> SNASKEKREKLEAYQHLFYLLQTNPTYLAKLIFQMPQNKSTKFMDSVIFTLYNYASNQREEYLLLRLFKTALQEEIKSKVDQIQEIVTGNPTVIKMVVSFNRGARGQNALRQILAPVVKEIMDDKSLNIKTDPVDIYKSWVNQMESQTGEASKLPYDVTPEQALAHEEVKTRLDSSIRNMRAVTDKFLSAIVSSVDKIPYGMRFIAKVLKDSLHEKFPDAGEDELLKIIGNLLYYRYMNPAIVAPDAFDIIDLSAGGQLTTDQRRNLGSIAKMLQHAASNKMFLGDNAHLSIINEYLSQSYQKFRRFFQTAC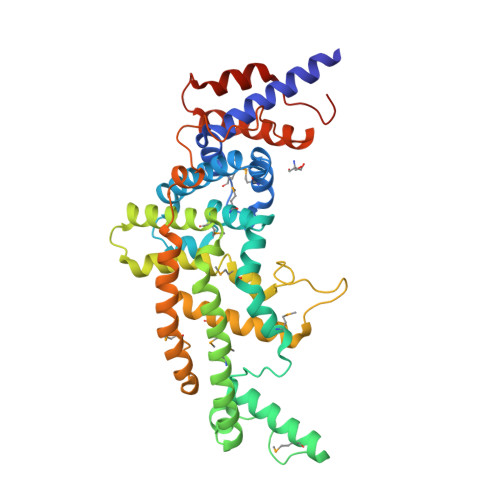DVPELQDKFNVDEYSDLVTLTKPVIYISIGEIINTHTLLLDHQDAIAPEHNDPIHELLDDLGEVPTIESLIGESS>MAHHHHHHMSAYVIDAAERPSVEVDQSSARFPVRRVF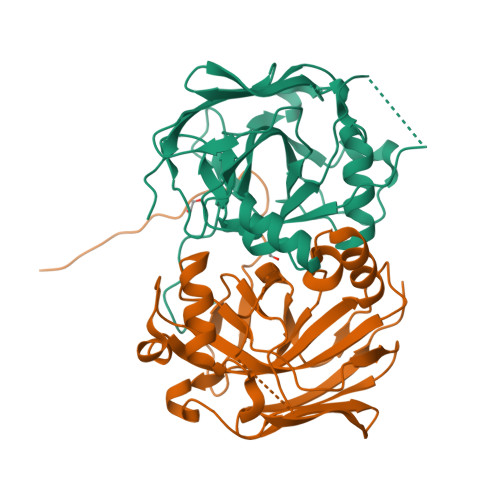CVGRNYADHAREMGADPDREPPFFFTKPADAIVPASGTVAYPPLTNDLHHEIELVVAIGKDGRSIDPADALSHVWGYGVGVDLTRRDLQAEAKKLSRPWDWAKGFDASGPVTALRAATATGHPAAGRIWLAVNGDTRQQGDLADMIWPVPDVIAYVSRSVELKAGDLIFTGTPAGVGALQPGDRVTGGVDGIATFEFVVGAKP[2x]>MISKEYHIDEEVGFALPNPQENLPDFYNDWMFIAKHLPDLIESGQLRERVEKLNMLSIDHLTDHKSQRLARLVLGCITMAYVWGKGHGDVRKVLPRNIAVPYCQLSKKLELPPILVYADCVLANWKKKDPNKPLTYENMDVLFSFRDGDCSKGFFLVSLLVEIAAASAIKVIPTVFKAMQMQERDTLLKALLEIASCLEKALQVFHQIHDHVNPKAFFSVLRIYLSGWKGNPQLSDGLVYEGFWEDPKEFAGGSAGQSSVFQCFDVLLGIQQTAGGGHAAQFLQDMRRYMPPAHRNFLCSLESNPSVREFVL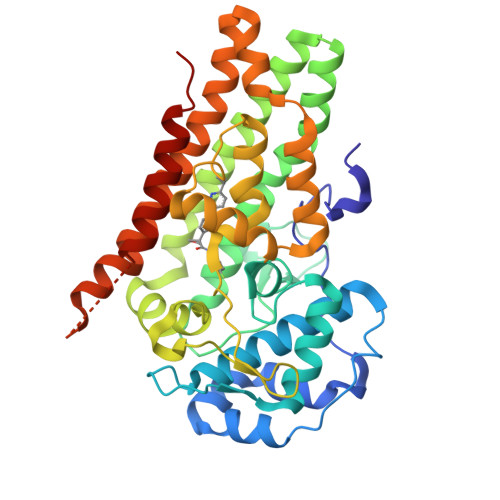SKGDAGLREAYDACVKALVSLRSYHLQIVTKYILIPASQQPKENKTSEDPSKLEAKGTGGTDLMNFLKTVRSTTEKSLLKEG[2x]>MSPKLPQHGTVGVRTPLVDGVEKVTGKAKYTADIAAPDALVGRILRSPHAHARILAIDTSAAEALEGVIAVCTGAETPVPFGVLPIAENEYPLARDKVRYRGDPVAAVAAIDEVTAEKALALIKVDYEVLPAYMTPKAAMKAGAIALHDDKPNNILREVHAEFGDVAAAFAEADLIREKTYTFAEVNHVHMELNATLAEYDPVRDMLTLNTTTQVPYYVHLKVAACLQMDSARIRVIKPFLGGGFGARTEALHFEIIAGLLARKAKGTVRLLQTREETFIAHRGRPWTEVKMKIGLKKDGKIAALALEATQAGGAYAGYGIITILYTGALMHGLYHIPAIKHDAWRVYTNTPPCGAMRGHGTVDTRAAFEALLTEMGEELGIDSLKIRQINMLPQIPYVTMYAQRVMSYGVPECLEKVKAASGWEERKGKLPKGRGLGIALSHFVSGTSTPKHWTGEPHATVNLKLDFDGGITLLTGAADIGQGSNTMASQVAAEVLGVRLSRIRVISADSALTPKDNGSYSSRVTFMVGNASISAAEELKGVLVKAAAKKLDAREEDIEVIDEMFMVSGSQDPGLSFQEVVKAAMVDSGTITVKGTYTCPTEFQGDKKIRGSAIGATMGFCYAAQVVEASVDEITGKVTAHKVWVAVDVGKALNPLAVEGQTQGGVWMGMGQALSEETVYDNGRMVHGNILDYRVPTIVESPDIEVIIVESMDPNGPFGAKEASEGMLAGFLPAIHEAVYEAVGVRATDFPLSPDRITELLDAKEAAA[2x];>[2x]MNILTDFRTHRPATLADAVNALAAEATLPLGAGTDLLPNLRRGLGHPAALVDLTGIDGLATISTLADGSLRIGAGATLEAIAEHDAIRTTWPALAQAAESVAGPTHRAAATLGGNLCQDTRCTFYNQSEWWRSGNGYCLKYKGDKCHVIVKSDRCYATYHGDVAPALMVLDARAEIVGPAGKRTVPVAQLFRESGAEHLTLEKGELLAAIEVPPTGAWSAAYSKVRIRDAVDFPLAGVAAALQRDGDRIAGLRVAITGSNSAPLMVPVDALLGGNWDDAAAETLAQLVRKTSNVLRTTITGVKYRRRVLLAISRKVVDQLWEAR;>[2x]MKNILRLTLNGRAREDLVPDNMLLLDYLRETVGLTGTKQGCDGGECGACTVLVDDRPRLACSTLAHQVAGKKVETVESLATQGTLSKLQAAFHEKLGT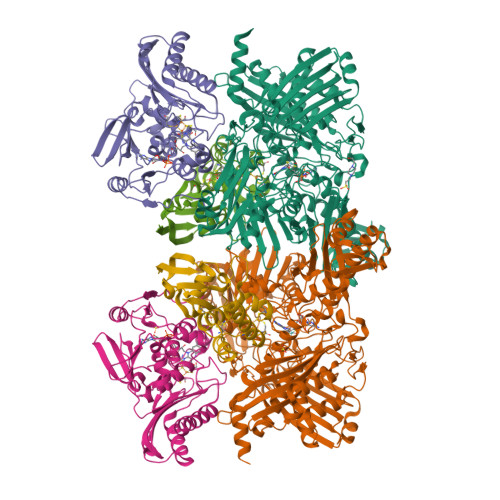QCGFCTPGMIMASEALLRKNPSPSRDEIKAALAGNLCRCTGYVKIIKSVETAAAARLCEEGAR> FSELLDLVGGLGRFQVLQTMALMVSIMWLCTQSMLENFSAAVPSHRCWAPLLDNSTAVSTSLSPEALLAISIPPGPNQRPHQCRRFRQPQWQLLDPNATATSWSEADTEPCVDGWVYDRSIFTSTIVAKWNLVCDSHALKPMAQSIYLAGILVGAAACGPASDRFGRRLVLTWSYLQMAVMGTAAAFAPAFPVYCLFRFLLAFAVAGVMMNTGTLLMEWTAARARPLVMTLNSLGFSFGHGLTAAVAYGVRDWTLLQLVVSVPFFLCFLYSWWLPESARWLIIKGKPDQALQELRKVARINGHKEAKNLTIEVLMSSVKEEVASAKEPRSVLDLFCVPGLRFRTCISTLCWFAFGFTFFGLALDLQALGSNIFLLQMFIGVVDIPAKMGALLLLSHLGRRPTLAASLLLAGLCILANTLVPHEMGALRSALAVLGLGGVGAAFTCITIYSSELFPTVLRMTAVGLGQMA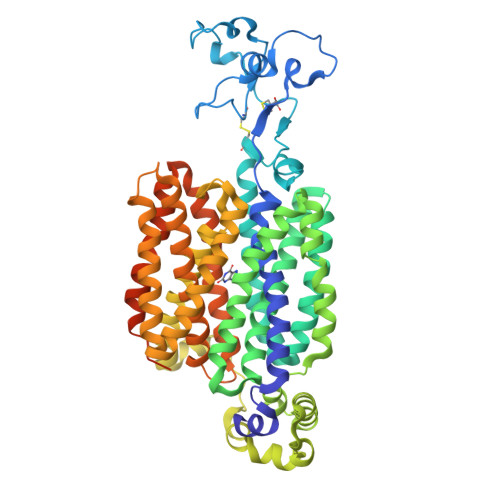ARGGAILGPLVRLLGVHGPWLPLLVYGTVPVLSGLAALLLPETQSLPLPDTIQDVQNQAVKKATHGTLGNSVLKSTQF N-terminal cysteine oxidases (NCOs) act as enzymatic oxygen (O2) sensors, coordinating cellular changes to hypoxia in animals and plants. They regulate the O2-dependent stability of proteins bearing an N-terminal cysteine residue through the N-degron pathway. In animals, the Cys branch of the N-degron pathway is regulated by the NCO 2-aminoethanethiol dioxygenase (ADO), which also plays a role in cysteamine catabolism and taurine biosynthesis. Biochemically, ADO is a non-haem iron-dependent thiol dioxygenase (TDO) from the cupin fold family of enzymes, consisting of a conserved double stranded β-helix (DSBH) core in which the active site is situated.

Following successful implementation of this strategy in generating a structure of ADO in complex with a substrate analogue, additional moieties were installed onto CP6 to examine interactions with extended pseudo-N-terminal sequences. CP6-L8 was replaced with 2,3-diaminopropionic acid (Dap; d), an amino acid that contains a sidechain amine linked to one carbon, from which the dipeptides Lys-Ser, Phe-Ser, and Gly-Ser were appended, to mimic the N-termini of known NCO substrates (RGS4/5, IL32, and RAP2 [an NCO target in plants,10], respectively; Fig. 3c). The pseudo-Nt-Ser residue remains coordinated to the metal centre in a bidentate arrangement, supported by interactions with ADO-F101, -D206 and -Y212, with one water molecule trans to ADO-H112, analogous to CP6-L8K-Ser. No additional interactions are observed except, possibly, weak water-mediated hydrogen bonds between the second amide of CP6-L8d-Gly-Ser and the sidechain hydroxyls of ADO-Y212 and -Y222, as these water molecules are absent in the CP6-L8K-Ser structure. The crystal structures of cobalt-incorporated ADO in complex with CP6-L8K-Ser and CP6-L8d-Gly-Ser provide valuable information on substrate analogue binding. However, they do not reflect native conditions in which an iron cofactor interacts with an Nt-Cys residue. To corroborate that the crystal structures of cobalt-incorporated ADO in complex with CP6-L8K-Ser and CP6-L8d-Gly-Ser are biologically relevant, molecular dynamic (MD) simulations were conducted with different combinations of active site metal and pseudo-N-terminal substrate residues over 100 ns. In each instance, no changes in hydrogen bonding distance were observed, with Ser and Cys interacting with cobalt(II) and iron(II) through ligation of both their amine and hydroxyl/thiol groups, supporting bidentate coordination of the substrate. MD was also used to calculate the binding energies associated with CP6-L8d-Gly-Ser/Cys complex formation, verifying key residue interactions, most notably the contributions of ADO-Y87 and CP6-W7, ADO-W257 and CP6-C14, ADO-Y212 and CP6-L8d-Gly-Ser/Cys, all of which were highlighted above during assessment of the crystal structure. It also emphasised the role of ADO-Q252, which forms hydrogen bonds with the backbone nitrogen and oxygen of CP6-R12.

> SMPRDNMASLIQRIARQASLTFRGSGGGRGASDRDAASGPEAPMQPGFPENLSKLKSLLTQLRAEDLNIAPRKATLQPLPPNLPPVTYMHIYETDGFSLGVFLLKSGTSIPLHDHPGMHGMLKVLYGTVRISCMDKLDAGGGQRPRALPPEQQFEPPLQPREREAVRPGVLRSRAEYTEASGPCILTPHRDNLHQIDAVEGPAAFLDILAPPYDPDDGRDCHYYRVLEPVRPKEASSSASDLPREVWLLETPQADDFWCEGEPYPGPKVFP;> XYIVKTFWSGSHRQCX6-[3-(1-adamantyl)-4-oxidanyl-phenyl]naphthalene-2-carboxylic 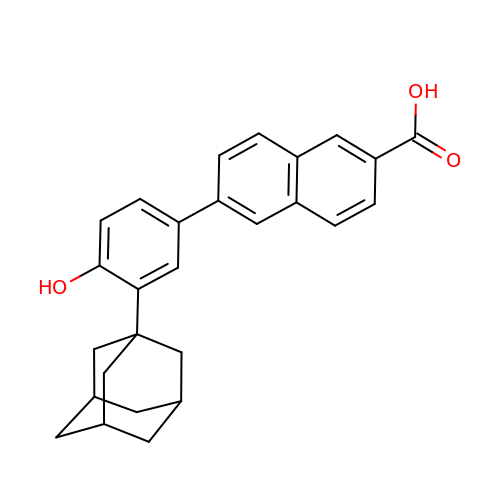acid | C27 H26 O3 | LDGIHZJOIQSHPB-HYVKCOOLSA-N> MTAPEQTFRNKKQRKQQVKLRKPGFAVAKYVRMSPRKVRLVVDVIRGKSVQDAEDLLRF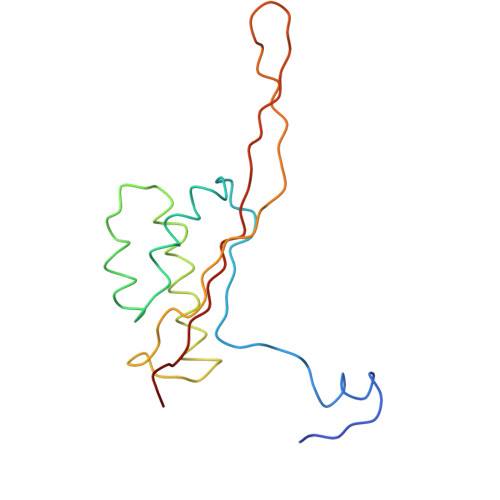IPRSASEPVAKVLNSAKANALHNDEMLEDRLFVKEAYVDAGPTLKRLIPRARGSANIIKKRTSHITIIVAEKGNK> MLSRKIIEESDIYLATSTRDPELFPLVIDHGEGVWIYDVDGNKYLDFTSGIGVNNLGWPSHPEVIKIGIEQMQKLAHAAANDFYNIPQLELAKKLVTYSPGNFQKKVFFSNSGTEAIEAS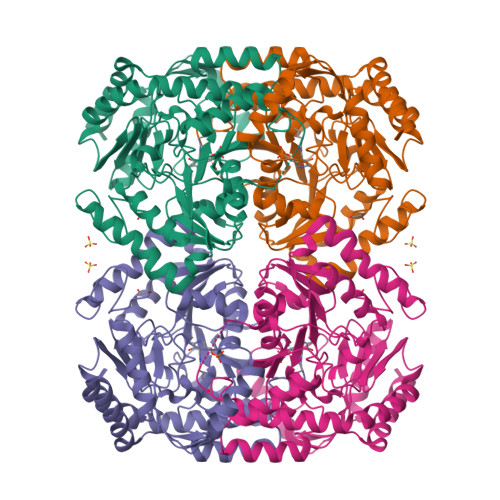IKVVKNTGRKYIIAFLGGFHGRTFGSISLTASKAVQRSIVGPFMPGVIHVPYPNPYRNPWHINGYENPSELVNRVIEFIEDYIFVNLVPPEEVAGIFFEPIQGEGGYVIPPKNFFAELQKLAKKYGILLVDDEVQMGLGRTGKLFAIENFNTVPDVITLAKALGGGIMPIGATIFRKDLDFKPGMHSNTFGGNALACAIGSKVIDIVKDLLPHVNEIGKIFAEELQGLADDVRGIGLAWGLEYNEKKVRDRIIGESFKRGLLLLPAGRSAIRVIPPLVISEEEAKQGLDILKKVIKVVK> SNAMLQFSF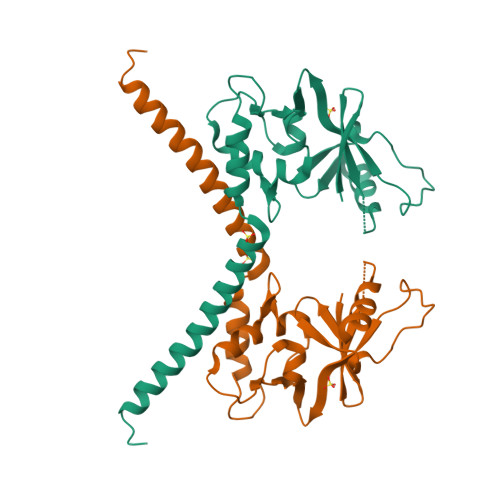VSNDVVMTYDGDSGEQIIWVWESLNKFQTVCISRIFNFQLQDLRNPPSTVQDFNDYEYSFNFGTLNNEYITVPGRILSINRDVLIHKSIKLERKVFASERNVSIFGRLSKLLDHTNPIIIGGDKPEAIPKSVFQELQSKFPNTGELDRYANARVHAILAGYLDGMKDARERYEHYLNRKTVI Each protein forms key interactions to promote cell infection, with the terminal domain of the fiber, the fiber knob protein, interacting with the viruses’ primary cell entry receptor. The adenovirus fiber knob protein is known to have a highly conserved trimeric structure. Sialic acid (SA) usage has been proposed as a cell infection mechanism for EKC causing HAdV-D. Here we highlight an important role for SA engagement by many HAdV-D. We provide apo state crystal structures of 7 previously undetermined HAdV-D fiber-knob proteins, and structures of HAdV-D25, D29, D30 and D53 fiber-knob proteins in complex with SA. Our findings demonstrate a conserved binding site for sialic acid, common across the species D adenoviruses, therefore suggesting that, along with CAR, the receptor can be used to initiate cell entry.

We performed X-ray crystallography to generate structures of species D human adenovirus fiber knob proteins HAdV-D15, D24, D29, D30, D32 and D53 in their apo states. HAdV-D53 is of particular interest due to the recent confirmation of EKC causing infection, similar to previously identified sialic acid binding viruses HAdV-D37 and D64. The fiber knob protein of HAdV-D53 was also investigated for its ability to interact with CAR. An accurate IC50 value could not be measured due to a lack of ability to block CAR antibody binding, even at the highest doses tested. Fiber-knob proteins of HAdV-D24, D26 and D32 all had a much weaker IC50 value, with HAdV-D53’s fiber-knob protein seemingly unable to interact with CAR. This again suggested a range of variability, with some viruses such as HAdV-D53 having a clear preference for sialic acid primarily but others demonstrating the ability to interact with both receptors. The species D adenoviruses are notable for their frequent recombination events and when investigated, HAdV-D53 seemed to have arisen from HAdV-D22 recombining with two sialic acid binding, EKC causing adenoviruses: HAdV-D8 and D3728,29. This recombination event, combining two viruses with similar tropisms explains our findings that HAdV-D53 appears to rely heavily on sialic acid as a cell entry receptor.

>KNNDKLTLWTTPDTSPNCRIDQDKDSKLTLVLTKCGSQILANVSLIVVAGRYKIINNNTNPALKGFTIKLLFDKNGVLMESSNLGKSYWNFRNQNSIMSTAYEKAIGFMPNLVAYPKPTTGSKKYARDIVYGNIYLGGKPHQPVTIKTTFNQETGCEYSITFDFSWAKTYVNVEFETTSFTFSYIAQE[6x]>[2x]QCVKLNDGHFMPVLGFGTYAPPEVPRSKALEVTKLAIEAGFRHIDSAHLYNNEEQVGLAIRSKIADGSVKREDIFYTSKLWSTFHRPELVRPALENSLKKAQLDYVDLYLIHSPMSLKPGEELSPTDENGKVIFDIVDLCT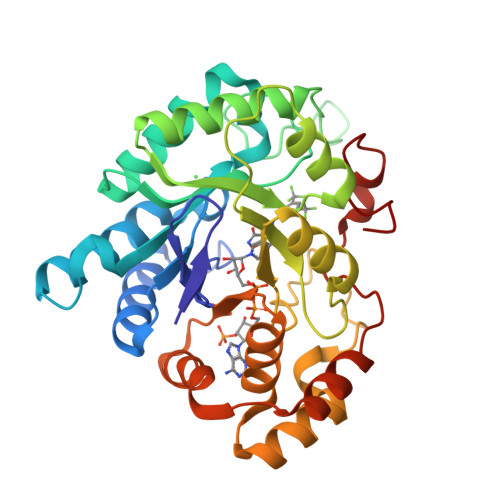TWEAMEKCKDAGLAKSIGVSNFNRRQLEMILNKPGLKYKPVCNQVECHPYFNRSKLLDFCKSKDIVLVAYSALGSQRDKRWVDPNSPVLLEDPVLCALAKKHKRTPALIALRYQLQRGVVVLAKSYNEQRIRQNVQVFEFQLTAEDMKAIDGLDRNLHYFNSDSFASHPNYPYSDEY>MNFRTLPDGVSAEQFANAISEFSETIGSEYVRVDEATVSEYDDKFPVTDGDEFKGSAVIWPGSTEDVQVIVRIANKYGIPLHAFSGGRNLGYGGSSPMLTGTVLLHLGKRMNRVLEINEKLAYAVVEPGVDYKTLYEAVRDSGAKLMIDPAELDWGSVMGNTMEHGVGYTPYADHSMWRCGMEVVLADGEVLRTGMGGLPGSEAWHLYPGQLGPSIEGLFEQSNFGICTRMGMQLMPTPPEMLSFAIYFENEDDLPAIMETTLPLRIGMAPLQAAPIVRNVTFDAACVSKREEWQTE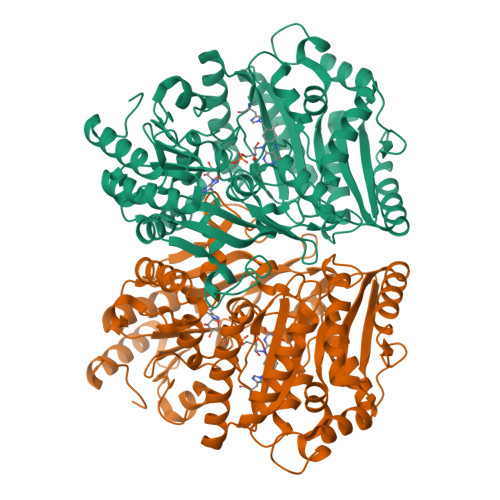PGPLTDEAKQRMVDELGIGHWIVYGTCYGPRWQIDKYIEMIRDAYLQIPGARFETNETLPLREGDRASELLNARHELNTGVPNRHSAAVFDWFPNAGHFFYAPVSAPSGEDAAKQYEDTKRISDDHGIDYLAQFIIGLREMHHICLPLYDTADPASRKETLDMTRELIRAGAEEGYGIYRAHNVLADQVAETYSFNNHIQRRSHERIKDALDPNGILNPGKSGIWPERLRNK[2x]>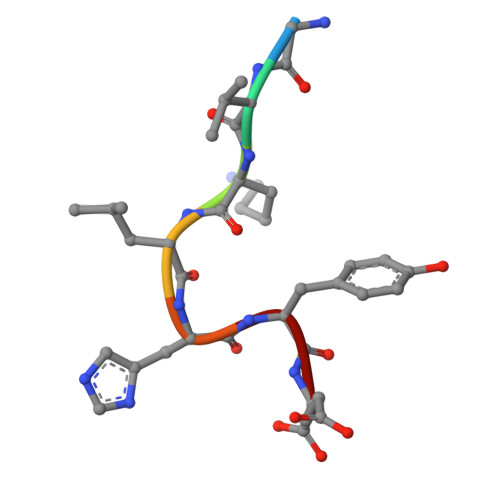 GVKLHYE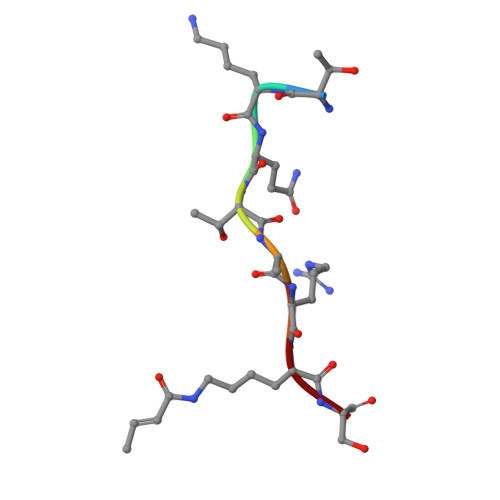> TKQTARXS>[8x]ATRSPGVVISDDEPGYDLDLFCIPNHYAEDLERVFIPHGLIMDRTERLARDVMKEMGGHHIVALCVLKGGYKFFADLLDYIKALNRNSDRSIPMTVDFIRLKSYCND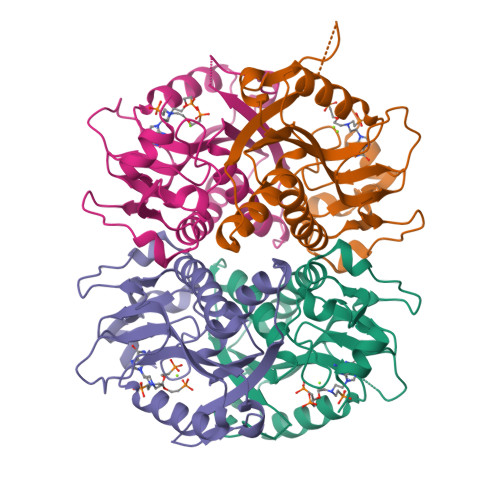QSTGDIKVIGGDDLSTLTGKNVLIVEDIIDTGKTMQTLLSLVRQYNPKMVKVASLLVKRTPRSVGYKPDFVGFEIPDKFVVGYALDYNEYFRDLNHVCVISETGKAKYKA>[6x]MPSNNRYDVTEWPAGNPAKDIGEVINSIIADIKARQGAADVDDGGKPGAVIYLPPGDYHLRTQVLIDISFLRIEGSGHGFTSSSIRFNVPEEEWPDLHELWPGGSRVIVDLPAGGAGDSAAGAAFLVAREGSPRISSVEFSNFCIDGLHFTADGSGRHPENTYANGKTGIHVASANDSFRVTDMGFVYLENALTIHKADALSIHHNFIAE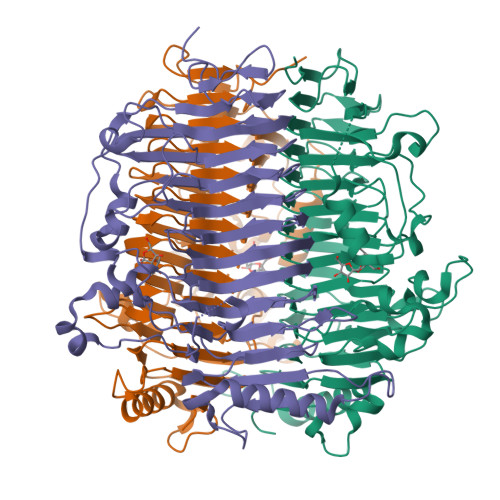CGSCIELRGWGQASKITDNLVGAGPRGHSIYAENHGGLLVTANNVFPRGASSVHFKGVTRSSVTNNRLHAFYPGMVRLEENSSENLVATNHFLRDHEPWTPFFGVDNGLDDLTGLLSISGNNNSVIGNHFSEVVDANEIRPEGATPVIIRLTAGTGNFVSTNHVVAMDVDAASSDSAFEAQVDALLATEAADLAVTAVLVDPGSARNTILDSGSDTQVVADRAVNAIRATPTVGF>[2x]MFNRLFRVCFLAALIMAFTLPNSVYAQKPIFKEVSVHDPSIIETNGTFYVFGSHLASAKSND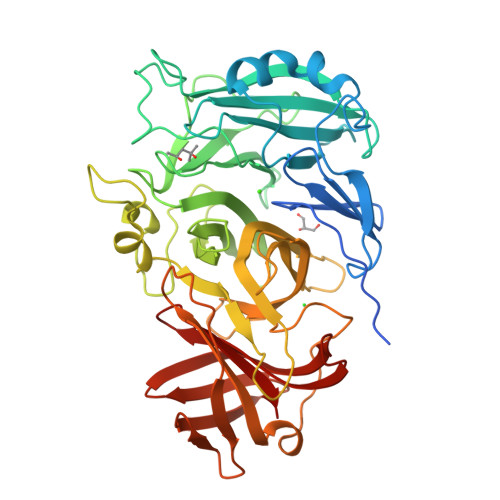LMQWQQLTTSVSNDNPLIPNVYEELKETFEWAQSDTLWAADVTQLADGKYYMYYNACRGDSPRSAMGVAVADNIEGPYKNKGIFLKSGMEGTSSDGTPYDATKHPNVVDPHTFFDKDGKLWMVYGSYSGGIFILEMNPKTGFPLPGQGYGKKLLGGNHSRIEGPYVLYNPDTQYYYLYLSYGGLDATGGYNIRVARSKKPDGPYYDAEGNPMLDVRGKGGTFFDDRSIEPYGVKLMGSYTFETENEKGTGYVSPGANSAYYDEKTGRSYLIFHTRFPGRGEEHEVRVHQLFMNKDGWPVAAPYRYAGETLKEVKQKDITGTYKLIQHGKDISADIKQTINIQLNKNHTISGEMTGTWRKTGKNTADITLAGKKYNGVFLRQWDSVREKNVMTFSVLNTSGEAVWGSKLA>[2x]MNLKALPAIEGDHNLKNYEETYRHFDWAEAEKHFSWHETGKLNAAYEAIDRHAESFRKNKVALYYKDAKRDEKYTFKEMKEESNRAGNVLRRYGNVEKGDRVFIFMPRSPELYFIMLGAIKIGAIAGPLFEAFMEGAVKDRLENSEAKVVVTTPELLERIPVDKLPHLQHVFVVGGEAESGTNIINYDEAAKQESTRLDIEWMDKKDGFLLHYTSGSTGTPKGVLHVHEAMIQQYQTGKWVLDLKEEDIYWCTADPGWVTGTVYGIFAPWLNGATNVIVGGRFSPESWYGTIEQLGVNVWYSAPTAFRMLMGAGDEMAAKYDLTSLRHVLSVGEPLNPEVIRWGHKVFNKRIHDTWWMTETGSQLICNYPCMDIKPGSMGKPIPGVEAAIVDNQGNELPPYRMGNLAIKKGWPSMMHTIWNNPEKYESYFMPGGWYVSGDSAYMDEEGYFWF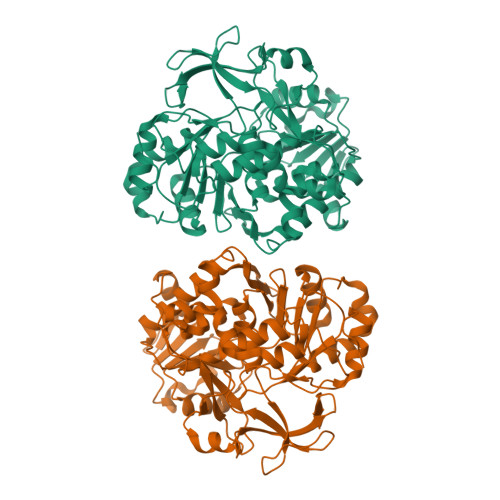QGRVDDVIMTSGERVGPFEVESKLVEHPAIAEAGVIGKPDPVRGEIIKAFIALREGFEPSDKLKEEIRLFVKQGLAAHAAPREIEFKDKLPKTRSGKIMRRVLKAWELNLPAGDLSTMED>[8x]HMEAVLYSTFRNHLKDYMKKVNDEFEPLTVVNKNPDEDIVVLSKSEWDSIQETLRIAQNKELSDKVLRGMAQVRA;>[4x]MLLKFTEDAWADYCYWQNQDKKTLKRINKLIKDIQR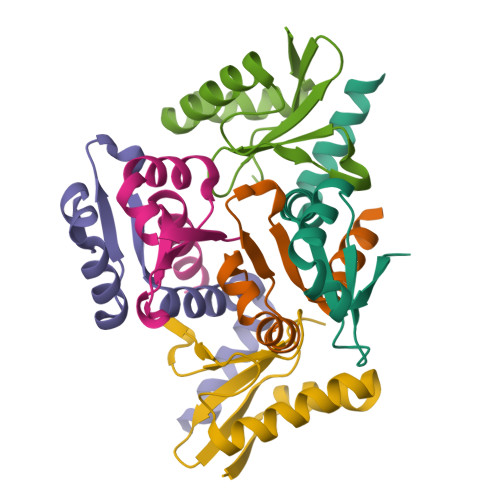DPFTGIGKPEPLKYDYQGAWSRRIDAENRLIYMMDGDSVAFLSFKDHY> MAAGVAAWLPFARAAAIGWMPVASG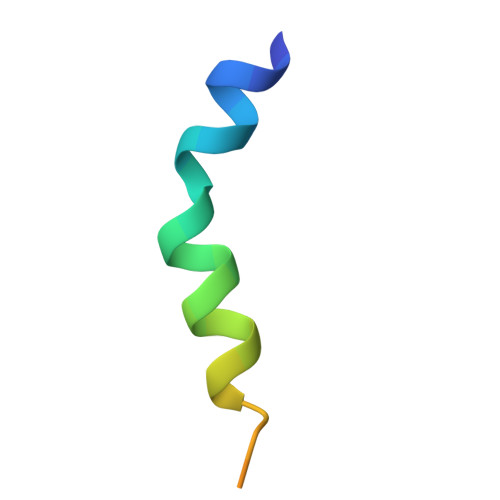PMPAP>MARILDGK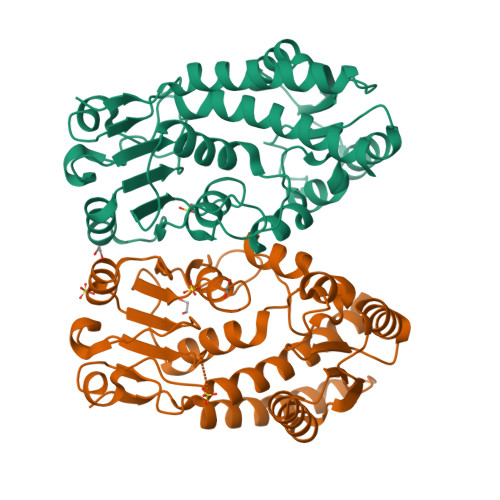ALAMEIKKELKQKIAQWVSLGNRAPTIRCIIVGDDPASHTYVRNKVEAAKFVGIDALTINRDSDITEEQLLSEIQNLNEDNSVDGILVQLPVPDTINERRVCDAIAPEKDIDGFHIINIGRLCVDLPTIVPATALAVVEMLKRFNIDTFGRNAVVIGRSKNVGMPIAMMLHSDKRHESGLGMDATVTICHRYTPKDKLEAYCRNADIIITATGLPKLIKADMVKPGATIIDVGITTRTDENGKSRLVGDVDYEEVSKIAGAITPVPGGVGPMTVAMLMHNTFQAAQSQANKSN[2x]> GAMCASRDDWRCARSMHEFSAKDIDGHMVNLDKYRGFVCIVTNVASQCGKTEVNYTQLVDLHARYAECGLRILAFPCNQF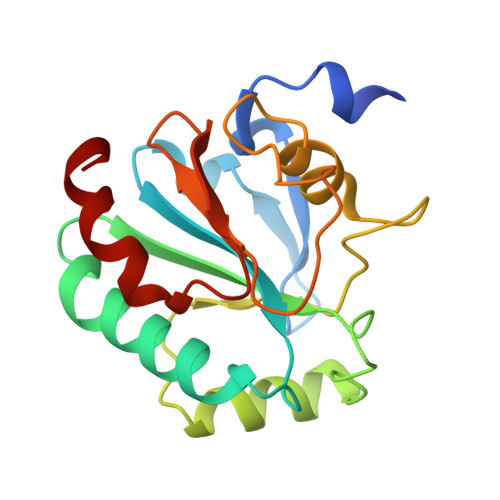GKQEPGSNEEIKEFAAGYNVKFDMFSKICVNGDDAHPLWKWMKIQPKGKGSSGNAIKWNFTKFLIDKNGCVVKRYGPMEEPLVIEKDLPHYF> VEYKNTICPPRQDYRYWYFVAELTIGVNYDINSTIIGECHMSESYIDRNANIVLTGYGLKINMTIMDTDQRFVAAAEGVGKDNK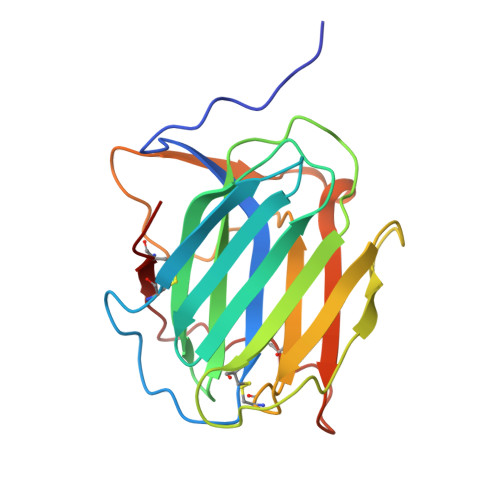LSVLLFTTQRLDKVHHNISVTITCMEMNCGTTKYNSDLPESIHKSSSCDITINGSCVTCVNLETDPTKINPHYLHPKNKYLYHNSEYSMRGSYGVTFIDELNQCLLDIKELSYDICYRE(2S,3R,4R,5S,6R)-3-(acetylamino)-4,5-dihydroxy-6-(hydroxymethyl)tetrahydro-2H-thiopyran-2-yl [(2R,3S,4R,5R)-5-(2,4-dioxo-3,4-dihydropyrimidin-1(2H)-yl)-3,4-dihydroxytetrahydrofuran-2-yl]methyl 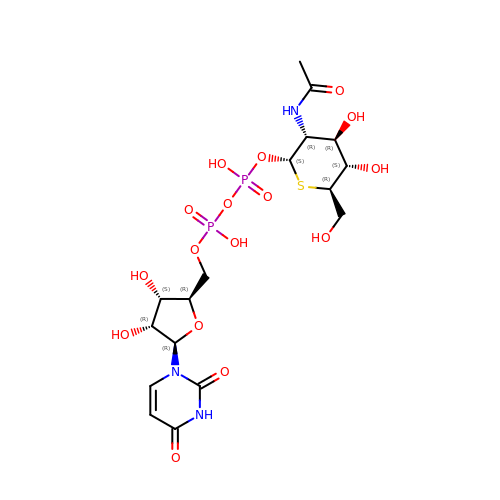dihydrogen diphosphate | C17 H27 N3 O16 P2 S | JPRVHSQHWXZSNC-UBDZBXRQSA-N>WSSHEQMLAQPLKDSDAEVYDIIKKESNRQRVGLELIASENFASRAVLEALGSCLNNKYSEGYPGQRYYGGTEHIDELETLCQKRALQAYGLDPQCWGVNVQPYSGSPANFAVYTALVEPHGRIMGLDLPDGGHLTHGFMTDKKKISATSIFFESMAYKVNPDTGYIDYDRLEENARLFHPKLIIAGTSCYSRNLDYGRLRKIADENGAYLMADMAHISGLVVAGVVPSPFEHCHVVTTTTHKTLRGCRAGMIFYRRGVRSVDPKTGKEILYNLESLINSAVFPGLQGGPHNHAIAGVAVALKQAMTPEFKEYQRQVVANCRALSAALVELGYKIVTGGS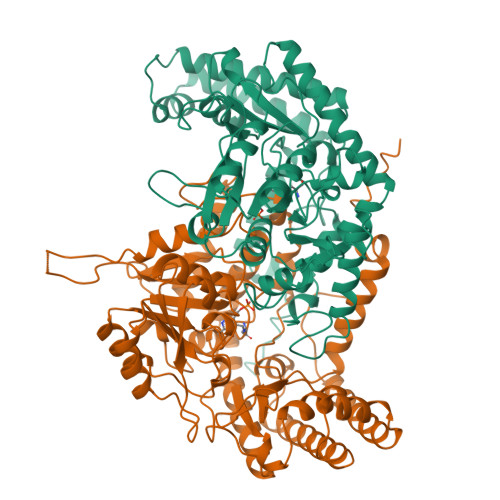DNHLILVDLRSKGTDGGRAEKVLEACSIACNKNTCPGDKSALRPSGLRLGTPALTSRGLLEKDFQKVAHFIHRGIELTVQIQDDTGPRATLKEFKEKLAGDEKHQRAVRALRQEVESFAALFPLPGLPGF[2x]>[2x]MSQFKNIIVTGGAGFIGSNFVHYVYNNHPDVHVTVLDKLTYAGNKANLEAILGDRVELVVGDIADAELVDKLAAKADAIVHYAAESHNDNSLNDPSPFIHTNFIGTYTLLEAARKYDIRFHHVSTDEVYGDLPLREDLPGHGEGPGEKFTAETNYNPSSPYSSTKAASDLIVKAWVRSFGVKATISNCSNNYGPYQHIEKFIPRQITNILAGIKP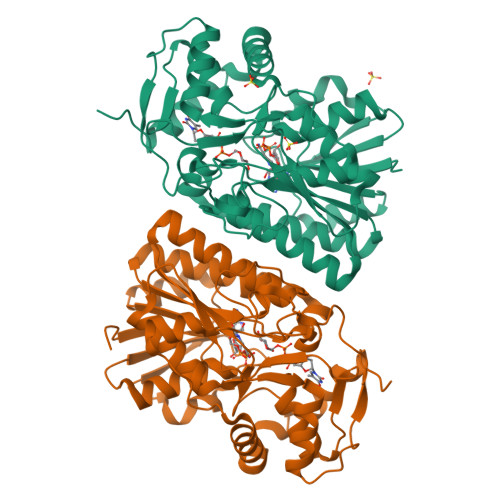KLYGEGKNVRDWIHTNDHSTGVWAILTKGRMGETYLIGADGEKNNKEVLELILEKMGQPKDAYDHVTDRAGHDLRYAIDASKLRDELGWTPQFTDFSEGLEETIQWYTDNQDWWKAEKEAVEANYAKTQEVIK>MTRTTGTRTTGILADGAIRALFAGDKLKSEADLDVDQVQPASLDLRLGSKAYRVRASFMPGPGTRVIDKLNRFSLHEVDLSQGAVLETGCVYIVPLMESLALPADMSASANPKSSTGRLDIFTRVMTDNAQEFDKIPAGYTGPLYLEISPRTFPIVVRRGSRLSQIRFRIGHALLNESEVLKLHETETLVASENPNVTGGGIALSIDLKGFGENGLIGYRGKHHTAVVDVDKKAQHDVLDFWEPLFARGRAELILDPDEFYILVSREAVHVPPLYAAEMTPFDPLVGEFRVHYAGFFDPGFGHAQAGGTGSRAVLEVRSHEVPFILEHGQIVGRLVYEHMLEKPEGLYGTGLGSNYQAQGLKLSKHFRAE[4x];> SN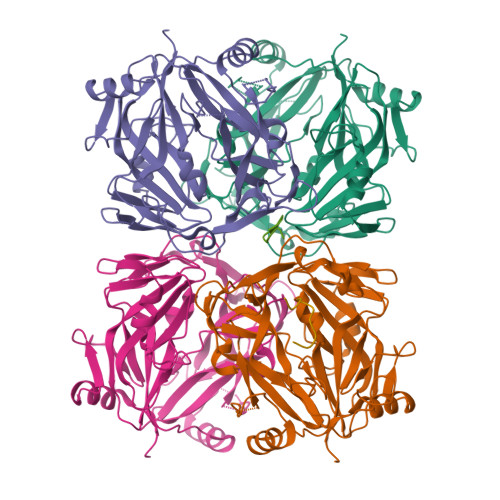PACVA;> VEVPLAGAV> TLSILVAHDLQRVIGFENQLPWHLPNDLKHVKKLSTGHTLVMGRKTFESIGKPLPNRRNVVLTSDTSFNVEGVDVIHSIEDIYQLPGHVFIFGGQTLYEEMIDKVDDMYITVIEGKFRGDTFFP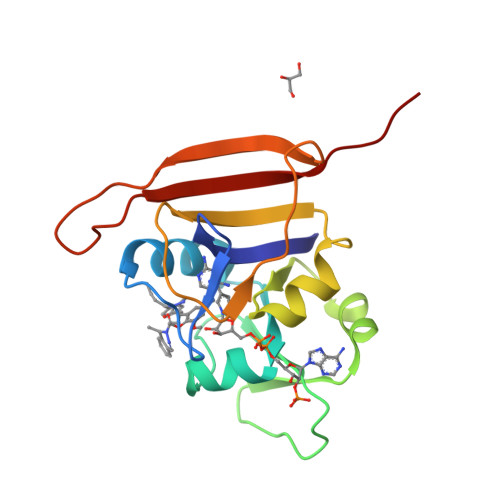PYTFEDWEVASSVEGKLDEKNTIPHTFLHLIRKAVPR>[2x]TADELVFFVNGKKVVEKNADPETTLLAYLRRKLGLRGTKLGCGEGGCGACTVMLSKYDRLQDKIIHFSANACLAPICTLHHVAVTTVEGIGSTKTRLHPVQERIAKSHGSQCGFCTPGIVMSMYTLLRNQPEPTVEEIEDAFQGNLCRCTGYRPILQGFRTFAK;>[2x]LFNPEEFMPLDPTQEPIFPPELLRLKDVPPKQLRFEGERVTWIQASTLKELLDLKAQHPEAKLVVGNTEIGIEMKFKNQLFPMIICPAWIPELNAVEHGPEGISFGAACALSSVEKTLLEAVAKLPTQKTEVFRGVLEQLRWFAGKQVKSVASLGGNIITASPISDLNPVFMASGTKLTIVSRGTRRTVPMDHTFFPSYRKTLLGPEEILLSIEIPYSREDEFFSAFKQASRREDDIAKVTCGMRVLFQPGSMQVKELALCYGGMADRTISALKTTQKQLSKFWNEKLLQDVCAGLAEELSLSPDAPGGMIEFRRTLTLSFFFKFYLTVLKKLG;>DTVGRPLPHLAAAMQASGEAVYCDDIPRYENELFLRLVTSTRAHAKIKSIDVSEAQKVPGFVCFLSADDIPGSNETGLFNDETVFAKDTVTCVGHIIGAVVADTPEHAERAAHVVKVTYEDLPAIITIEDAIKNNSFYGSELKIEKGDLKKGFSEADNVVSGELYIGGQDHFYLETHCTIAIPKGEEGEMELFVSTQNAMKTQSFVAKMLGVPVNRILVRVKRMGGGFGGKETRSTLVSVAVALAAYKTGHPVRCMLDRNEDMLITGGRHPFLARYKVGFMKTGTIVALEVDHYSNAGNSRDLSHSIMERALFHMDNCYKIPNIRGTGRLCKTNLSSNTAFRGFGGPQALFIAENWMSEVAVTCGLPAEEVRWKNMYKEGDLTHFNQRLEGFSVPRCWDECLKSSQYYARKSEVDKFNKENCWKKRGLCI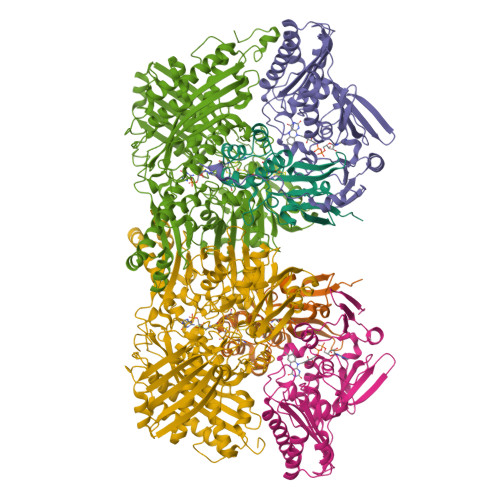IPTKFGISFTVPFLNQAGALIHVYTDGSVLVSHGGTEMGQGLHTKMVQVASKALKIPISKIYISETSTNTVPNSSPTAASVSTDIYGQAVYEACQTILKRLEPFKKKNPDGSWEDWVMAAYQDRVSLSTTGFYRTPNLGYSFETNSGNAFHYFTYGVACSEVEIDCLTGDHKNLRTDIVMDVGSSLNPAIDIGQVEGAFVQGLGLFTLEELHYSPEGSLHTRGPSTYKIPAFGSIPTEFRVSLLRDCPNKKAIYASKAVGEPPLFLGASVFFAIKDAIRAARAQHTNNNTKELFRLDSPATPEKIRNACVDKFTTLCVTGAPGNCK[2x]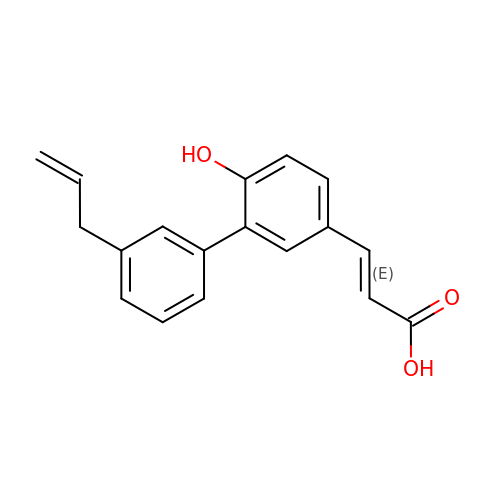(2E)-3-[6-hydroxy-3'-(prop-2-en-1-yl)biphenyl-3-yl]prop-2-enoic acid | C18 H16 O3 | RHYATHLMUIVCPK-CSKARUKUSA-N>[3x]SDAQEILSRLNSVLEAAWKTILNLASATDAAEKAYKEGREEDLATY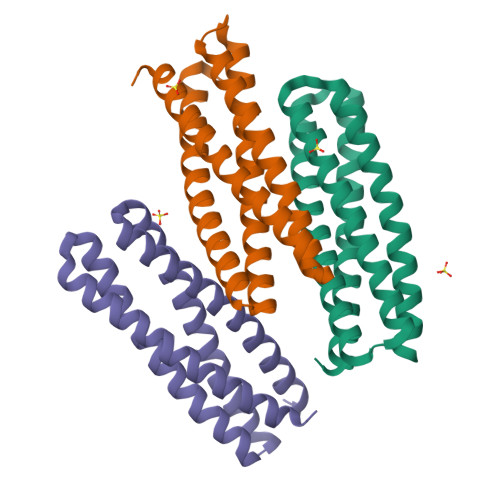LDQAASYQSQVDQYAVETVRLLAELKKVFPDEEADRALQIAEKLLKTVQEASKTLDTAVAAAANGDEETFAKAFNQFVSLGNQADTLFTQLQRTLTNLNKK>MGSSHHHHHHHQRMIIVDNNKLNVRALPSFIDYFNGIYGFATGIKDIMGMIFKTDTGGSNLTLDEILKNQNLLNDISGKLDGINGDLGDLIAQGNLNSELAKELLKISNEQNQMLNHVNAQLNAINSTLNIYLPKITSMLNEVMKQNHVLSLQIEFLSKQLQEISDKLDIINLNVLINSTLTEITPAYQRIKYVNEKFDELTSTVEKNPKSYQDNVTKEVIENLNELTELAKSVTKNDMDSFEFYLQTFHDVMTGNNLFGRSALKTASELITKENVTTRGSEIGKVYNFLIVLTSLQAKAFLTLTACRKLLGLTDIDYTQIMNHHIDGQKREFRINILPTLSNNFSNPSYSKNRGSDIDDPIVVLEAAPGYALIGFEILNDPLPILKGYQARLKPNYQVDRESMSETIYGDIHKLFCPKQLEQKYYIKDIEFPEGYVITKIVFEKRLNQLGYEVTANFYDPSTGSIDLNKVKVESSSCEDEYSIIKAETDGIYMPLGVVSETFLTPIYGFGLTVDAANAAITLTGKSYLRESLLETDLLNNETYLIASPDGYISSIVENWNITSDNTGSWRANNNNAFVDKAGSSSLYTHKDGEFSQFIGNKLKPKTNYVIQYVIKGRPAIYLKNNKDTLFEDTKNNFSDFQ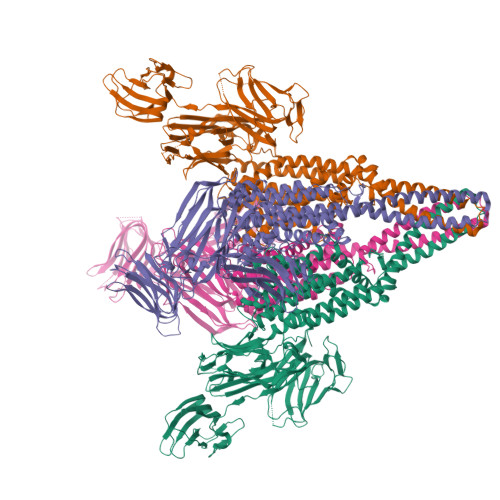TVTKKFNSGVNPSEIYFLFKNQSEYEAWGNNFIILEIKSLEFLPQMLKPEDWIPSGNVQMKDGGRLEILGDGYFKQFIKLENDSTYHLRLSVKGTGRVSIIDESKYLLFVNVKDEDLTRVIKNTSSKGECFIALEGTYVENSSTIFSNVSIVKE[4x]> MHHHHHHS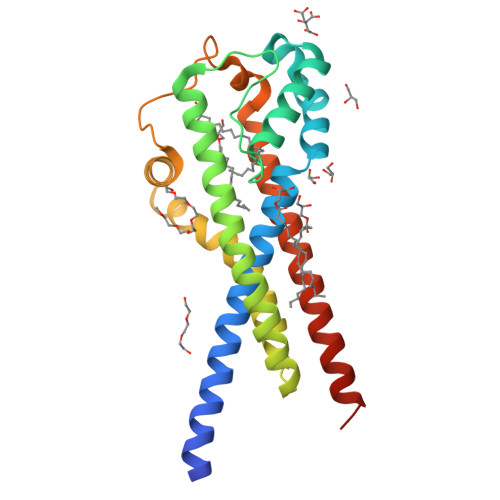SGRENLYFQGHMDRLITLVVSYSIAFSIFALATMAVVYGKWLYYFEIDFLNIPDLADMTKDEIKRNYDVLITYLSPFYDGALHLPTLDMSTNGRIRFVDVKNILVKIQYVMYATIMIAVIGGIYLLKKKNEKFLLHGSILTIIFPIALMLPIAINFEKSFVLFHKLLFSNDYWVFDPEKDPIILMLPEEFFMHAACAILLFILGGSILCYSLYRYLVKKKRMSQKKFSA Type 4 pili (T4P) are retractable surface appendages found on numerous bacteria and archaea that play essential roles in various microbial functions, including host colonization by pathogens. T4P are composed of thousands of copies of a major pilin protein arranged in a helical array. They are assembled and retracted by a complex machine composed of several essential proteins, including a dedicated extension ATPase, most often called PilB, that is essential for pilus biogenesis. Here, we report the cryo-electron microscopy (cryo-EM) structure of the BfpD ATPase from enteropathogenic Escherichia coli (EPEC) in the presence of either ADP or a mixture of ADP and AMP-PNP. Both structures, solved at 3 Å resolution, reveal the typical toroid shape of AAA+ ATPases and unambiguous 6-fold symmetry.

Purified BfpD was prepared under two nucleotide conditions: either in the presence of ADP (BfpD-ADP data set) or in the presence of ADP, ATP, and the nonhydrolysable ATP analog, AMP-PNP (termed BfpD-ANP data set) at a ratio of 2:4:5. After confirming structural integrity of the sample, cryo-EM and high-throughput data collection yielded 7,207 good movies and 313,223 good particles for BfpD-ADP. Subsequent 3D reconstruction with C6 symmetry yielded resolutions of 3.1 Å, 3.0 Å, and 3.7 Å for BfpD-ADP, BfpD-ANP class-1 and BfpD-ANP class-2, respectively. Additionally, in the BfpD-ADP map, Mg2+ is seen between Ser267 (from the Walker A motif) and the beta-phosphate of ADP. The loop (294-310) carrying the catalytic Glu295 has a well-defined cryo-EM density and is positioned closer to the nucleotide in BfpD-ADP compared to BfpD-ANP, assisted by a hydrogen bond between ADP and Tyr296. Comparison of the BfpD-ADP and BfpD-ANP structures reveals a subtle outward shift in position of the N2D with respect to the CTD such that the mobile innermost N2D loops delineate a circle of 65 Å in diameter (distance between diagonally located Ala172 residues) in the presence of ADP, and 70–73 Å diameter in the presence of ANP class 1 and 2, respectively. This change is accompanied by a slight change in angle of 1.1° for the N2D and 1.6° for the CTD between each monomer and the vertical axis for the BfpD-ANP structure compared to the BfpD-ADP structure, which is consistent with the outward shift in the center of mass described in the much lower resolution TtPilB cryo-EM structure. Transition from BfpD-ADP to BfpD-ANP resulted in a slight outward shift of the top part of the toroid, a tendency more pronounced in BfpD-ANP class 2. Top and side view: As a result of N2D twisting in each of the six subunits, the BfpD ring contracts during the transition from ANP class-2 to ADP and vice versa. The ring closure represents an event of ATP-bound BfpD, progressing to the post-ATP hydrolysis state (ADP).

>MVNKTEKTSDLMFERFKRNVSEIVTGDGGELELTVEQRKYFLIFKNGDFLVSSCHMKHHLVQMLREIATRKGYPNLTIYEVNLKDIRLLYEASLKTVQNNGQDLLPVEKRASMLLFECAEMRVSDLHIKVYDAEADIYIRKDGDMELLRQIESNTAHSILASLYNNADDSDATYKINAYQAARIVASKSRLALPPVIQAVRLQFNPLGQGGRYLIARFLYTDKSEKQKEMDPTRFGFHHSHAESFSRMRNLPIGINIISGPTGSGKSTTLKNLLELLYIEKKKKVNIISIEDPPEYEIDGTAQLPITNVETEAQRGEEYRKAITAALRSDPDIIMPGEARDAEVINLLFTAAMTGHQVWTSLHANNALAIFDRLKDQGVDEFKLTDPELITGLVAQRLVRKLCAQCSITLTEYIASGGGISDTDRKIISGHETSVRFPNPRAKKCCRDGYNGRTILAEVIEPDSKLLRLVAEGKREDAQHYWLTSLHGMALKEHAWLKIISGEICVMDAVNKISGIDNITEERKKYLFSRDNEI[6x]>[2x]MSAERILVTGGAGFIGSHLV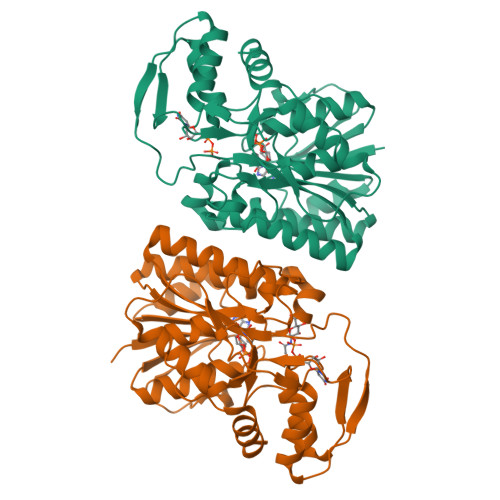DALLAKGYAVRVLDDLSTGKVGNLPMGDAGLELLVGDAADAALLADAVQGCDAVVHLAAVASVQASVEDPVATHQSNFIATLRLCEAMTAAGIRRVVFASAAAVYGNNGEGTPIAEDTPKSPLTPFAADKLASEYYLDFYRRQHGLEPVILRFFNIFGPRQDPSSPYSGVISIFSERAKAGRPITLFGDGGQTRDFVYVADLVKILVQGLESPAPAADATNVGLGGVTTLNDLIGALQQISGKPLQVSHGATRSGDIRHSKADNRRLRERFDLGTPSSLAEGLERLYRSL> MAGQAFRKFLPLFDRVLVERSA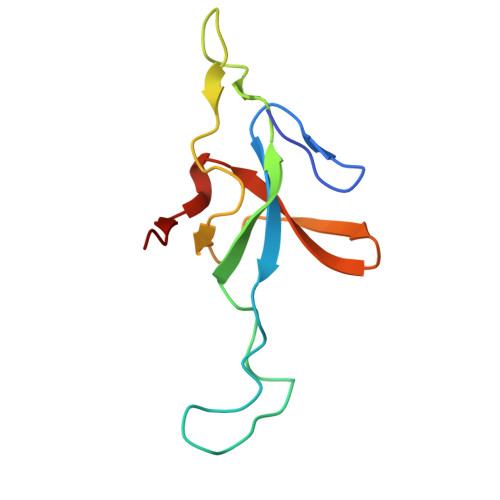AETVTKGGIMLPEKSQGKVLQATVVAVGSGSKGKGGEIQPVSVKVGDKVLLPEYGGTKVVLDDKDYFLFRDGDILGKYVD> MSYMLPHLHNGWQVDQAILSEEDRVVVIRFGHDWDPTCMKMDEVLYSIAEKVKNFAVIYLVDITEVPDFNKMYELYDPCTVMFFFRNKHIMIDLGTGNNNKINWAMEDKQEM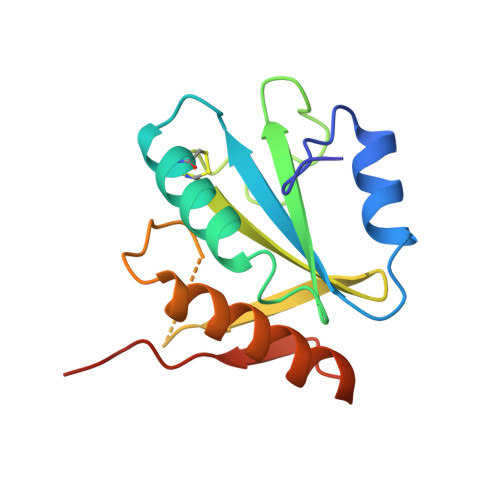VDIIETVYRGARKGRGLVVSPKDYSTKYRY> GHMHAPLVSKDLDYISTANHDQPPRHLGSRFSAEGEFLPEPGNTVVCHLVEGSQTESAIVSTRQRFLDMPEASQLAFTPVSSLHMTVFQGVIESRRALPYWPQTLPLDTPIDAVTDYYRDRLSTFPTLPAFNMRVTGLRPVGMVMKGATAEDDSIVALWRDTFADFFGYRHPDHDTYEFHITLSYIVSWFEPECLPRWQAMLDEELEKLRVAAPVIQMRPPAFCEFKDM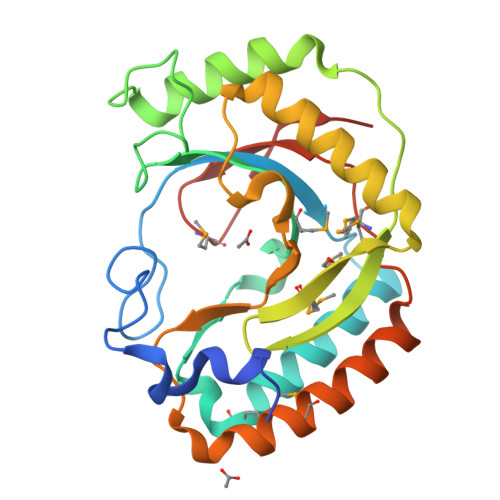NHFKELVVFDKRGS> SNAMSRIDDLQQDIESLLSEINSLEESREKLKAKIKDKRKNEESANPIVQEFEDLFDQFPQLNNFLFNEHPELEETDDKDISRAQADIPATPIPYEPKKRAKLENEEILPEQEWVLKTQPMVQHQMFDPGVADLLDTDILTSPSKRKRKLKIDDISTSDRSELEDYIVLENVYRMFGITFFPLVDPIDLKIKDASGEIFVDREMLGIRLEVFSERTSQFEKPHYVLLKKRIKSNSWFLFKHTIPSFIDVQGIFDDTNGGLVISHDDAYLFAKRVFLQLVEVQKRRQIFKDLEAKKIIHDLDLDLESSMVSFFVKDIKVELFVKQNEIVSCSILDDIHDFSQNNKSKWEIAL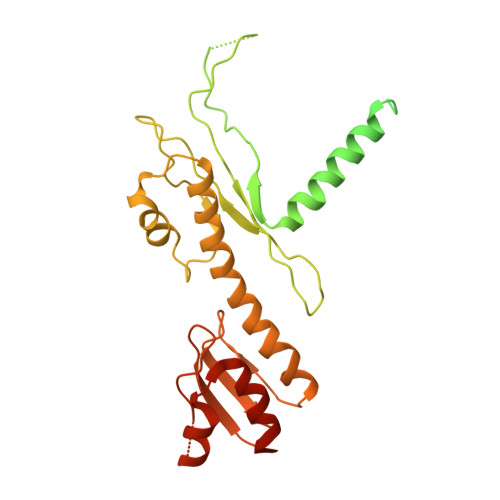LGSLDDLELKLNHSFATIFK> MGMKEKFVLIITHGDFGKGLLSGAEVIIGKQENVHTVGLNLGDNIEKVAKEVMRIIIAKLAEDKEIIIVVDLFGGSPFNIALEMMKTFDVKVITGINMPMLVELLTSINVYDTTE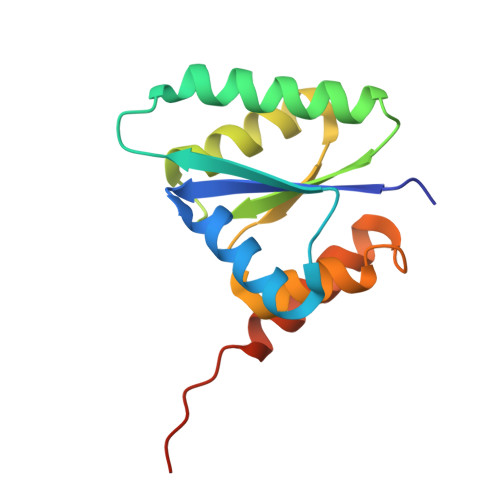LLENISKIGKDGIKVIEKSSLKM>MDKFRVQGPTRLQGEVTISGAKNAALPILFAALLAEEPVEIQNVPKLKDIDTTMKLLTQLGTKVERDGSVWIDASNVNNFSAPYDLVKTMRASIWALGPLVARFGQGQVSLPGGSAIGARPVDLHIFGLEKLGAEIKLEEGYVKASVNGRLKGAHIVMDKVSVGATVTIMSAATLAEGTTIIENAAREPEIVDTANFLVALGAKISGQGTDRITIEGVERLGGGVYRVLPDRIETGTFLVAAAISGGKIVCRNAQPDTLDAVLAKLREA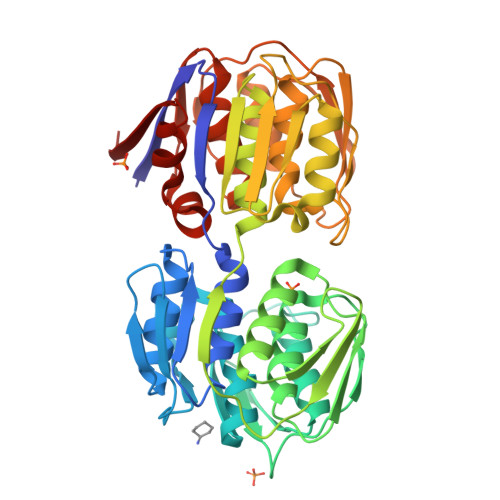GADIETGEDWISLDMHGKRPKAVTVRTAPHPAFPTDMQAQFTLLNLVAEGTGVITETIFENRFMHVPELIRMGAHAEIESNTVICHGVEKLSGAQVMATDLRASASLVLAGCIAEGTTVVDRIYHIDRGYERIEDKLRALGANIERVKGE[2x]Amongst the Arabidopsis MSL channels, MSL10 is enigmatic in that it has two separable functional modalities, regulated cell death signaling conferred by its N-terminal soluble ‘death’ domain and force-activated ion channel activity imparted by its C-terminal portion. When heterologously expressed in Xenopus oocytes, MSL10 is indeed activated by membrane stretch and displays a preference for anions. In Arabidopsis, MSL10 is primarily expressed in the shoot apex, root tips, and vascular tissues, playing a critical role in adaptation to hypo-osmotic shock and induction of programmed cell death. Analogous to DmMSL10/FLYC1, each subunit of the heptameric AtMSL10 channel is composed of a transmembrane domain (TMD) with six membrane-spanning helices (TM1-TM6) and a characteristic C-terminal cytoplasmic domain (CTD) shared by all MscS homologs.

Of particular interest, transient overexpression of the G556V mutation, near the helical kink in TM6, in tobacco epidermal cells resulted in a well-expressed protein as assessed by confocal imaging and the planta cell death assay. However, recordings from excised membrane patches showed no detectable currents of G556V under applied tension, indicating that the mutation stabilizes a non-conducting conformation. To better understand the open-to-closed transition of AtMSL10, we determined the cryo-EM structure of G556V at a nominal resolution of ~3.5 Å. The global structure of G556V is almost identical to that of the wild type (r.m.s.d of ~1.1 Å for all Cα atoms). Importantly, pronounced local conformational changes occur at the F553 hydrophobic gate, though the pore-lining helices align well with those of the wild type and the helical kinks are maintained. Introduction of a bulkier hydrophobic residue, valine, at the position of G556 pushes the aromatic side chain of F553 toward the central pore axis. Consequently, reorientation of the phenylalanine side chain reduces the pore radius from 6.6 to 3.9 Å at the position of the F553 ring, which is now remarkably similar to the dimension of the corresponding F572 ring in the wild-type DmMSL10/FLYC1 structure (3.5 Å in radius). Together with the lack of activating currents of the G556V variant in excised membrane patches, we conclude that this conformation represents a non-conducting, closed state. The wild-type AtMSL10 structure has a wide-open pore, whereas a non-conducting mutant G556V renders a much narrower pore created by repositioning of the side chain of F553, which appears to constitute the hydrophobic gate in the closed state. Closure of the channel pore could be essentially accomplished by local adjustment of the side chain of a critical residue defining the narrowest pore, while the global conformations of the open and closed states are similar.

>[7x]MAEQKSSNGGGGGGDVVINVPVEEASRRSKEMASPESEKGVPFSKSPSPEISKLVGSPNKPPRAPNQNNVGLTQRKSFARSVYSKPKSRFVDPSCPVDTSILEEEVREQLGAGFSFSRASPNNKSNRSVGSPAPVTPSKVVVEKDEDEEIYKKVKLNREMRSKISTLALIESAFFVVILSALVASLTINVLKHHTFWGLEVWKWCVLVMVIFSGMLVTNWFMRLIVFLIETNFLLRRKVLYFVHGLKKSVQVFIWLCLILVAWILLFNHDVKRSPAATKVLKCITRTLISILTGAFFWLVKTLLLKILAANFNVNNFFDRIQDSVFHQYVLQTLSGLPLMEEAERVGREPSTGHLSFATVVKKGTVKEKKVIDMGKVHKMKREKVSAWTMRVLMEAVRTSGLSTISDTLDETAYGEGKEQADREITSEMEALAAAYHVFRNVAQPFFNYIEEEDLLRFMIKEEVDLVFPLFDGAAETGRITRKAFTEWVVKVYTSRRALAHSLNDTKTAVKQLNKLVTAILMVVTVVIWLLLLEVATTKVLLFFSTQLVALAFIIVSTCKNLFESIVFVFVMHPYDVGDRCVVDGVAMLVEEMNLLTTVFLKLNNEKVYYPNAVLATKPISNYFRSPNMGETVEFSISFSTPVSKIAHLKERIAEYLEQNPQHWAPVHSVVVKEIENMNKLKMALYSDHTITFQENRERNLRRTELSLAIKRMLEDLHIDYTLLPQDINLTKKNSLEVLFQ> MAQALLVPPGPESFRLFTRESLAAIEKRAAEEKAKKPKKEQDNDDENKPKPNSDLEAGKNLPFIYGDIPPEMVSEPLEDLDPYYINKKTFIVMNKGKAIFRFSATSALYILTPLNPVRKIAIKILVHSLFSMLIMCTILTNCVFMTLSNPPDWTKNVEYTFTGIYTFESLIKILARGFCLEDFTFLRDPWNWLDFSVIVMAYVTEFVSLGNVSALRTFRVLRALKTISVIPGLKTIVGALIQSVKKLSDVMILTVFCLSVFALIGLQLFMGNLRNKCLQWPPSDSAFETNTTSYFNGTMDSNGTFVNVTMSTFNWKDYIGDDSHFYVLDGQKDPLLCGNGSDAGQCPEGYICVKAGRNPNYGYTSFDTFSWAFLSLFRLMTQDYWENLYQLTLRAAGKTYMIFFVLVIFLGSFYLVNLILAVVAMAYEEQNQATLEEAEQKEAEFQQMLEQLKKQQEEAQAVAAASAASRDFSGIGGLGELLESSSEASKLSSKSAKEWRNRRKKRRQREHLEGNNKGERDSFPKSESEDSVKRSSFLFSMDGNRLTSDKKFCSPHQSLLSIRGSLFSPRRNSKTSIFSFRGRAKDVGSENDFADDEHSTFEDSESRRDSLFVPHRHGERRNSNVSQASMSSRMVPGLPANGKMHSTVDCNGVVSLVGGPSALTSPTGQLPPEGTTTETEVRKRRLSSYQISMEMLEDSSGRQRAVSIASILTNTMEELEESRQKCPPCWYRFAN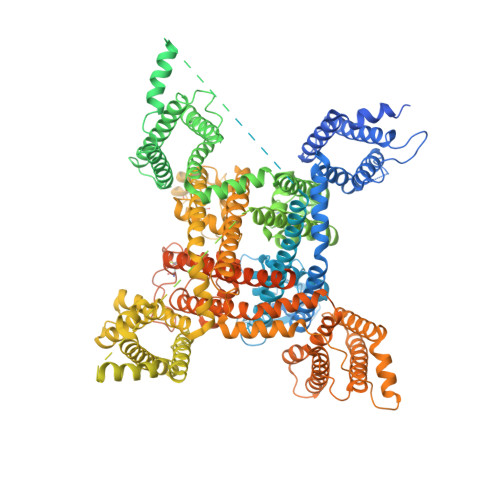VFLIWDCCDAWLKVKHLVNLIVMDPFVDLAITICIVLNTLFMAMEHYPMTEQFSSVLTVGNLVFTGIFTAEMVLKIIAMDPYYYFQEGWNIFDGIIVSLSLMELGLSNVEGLSVLRSFRLLRVFKLAKSWPTLNMLIKIIGNSVGALGNLTLVLAIIVFIFAVVGMQLFGKSYKECVCKINDDCTLPRWHMNDFFHSFLIVFRVLCGEWIETMWDCMEVAGQTMCLIVFMLVMVIGNLVVLNLFLALLLSSFSSDNLAATDDDNEMNNLQIAVGRMQKGIDYVKNKMRECFQKAFFRKPKVIEIHEGNKIDSCMSNNTGIEISKELNYLRDGNGTTSGVGTGSSVEKYVIDENDYMSFINNPSLTVTVPIAVGESDFENLNTEEFSSESELEESKEKLNATSSSEGSTVDVVLPREGEQAETEPEEDLKPEACFTEGCIKKFPFCQVSTEEGKGKIWWNLRKTCYSIVEHNWFETFIVFMILLSSGALAFEDIYIEQRKTIKTMLEYADKVFTYIFILEMLLKWVAYGFQTYFTNAWCWLDFLIVDVSLVSLVANALGYSELGAIKSLRTLRALRPLRALSRFEGMRVVVNALVGAIPSIMNVLLVCLIFWLIFSIMGVNLFAGKFYHCVNMTTGNMFDISDVNNLSDCQALGKQARWKNVKVNFDNVGAGYLALLQVATFKGWMDIMYAAVDSRDVKLQPVYEENLYMYLYFVIFIIFGSFFTLNLFIGVIIDNFNQQKKKFGGQDIFMTEEQKKYYNAMKKLGSKKPQKPIPRPANKFQGMVFDFVTRQVFDISIMILICLNMVTMMVETDDQGKYMTLVLSRINLVFIVLFTGEFVLKLVSLRHYYFTIGWNIFDFVVVILSIVGMFLAEMIEKYFVSPTLFRVIRLARIGRILRLIKGAKGIRTLLFALMMSLPALFNIGLLLFLVMFIYAIFGMSNFAYVKKEAGIDDMFNFETFGNSMICLFQITTSAGWDGLLAPILNSAPPDCDPDTIHPGSSVKGDCGNPSVGIFFFVSYIIISFLVVVNMYIAVILENFSVATEESAEPLSEDDFEMFYEVWEKFDPDATQFIEFSKLSDFAAALDPPLLIAKPNKVQLIAMDLPMVSGDRIHCLDILFAFTKRVLGESGEMDALRIQMEDRFMASNPSKVSYEPITTTLKRKQEEVSAAIIQRNFRCYLLKQRLKNISSNYNKEAIKGRIDLPIKQDMIIDKLNGNSTPEKTDGSSSTTSPPSYDSVTKPDKEKFEKDKPEKESKGKEVRENQK>[2x]MTHSQQSMVDTFRASLFDNQDITVADQQIQALPYSTMYLRLNEGQRIFVVLGYIEQEQSKWLSQDNAM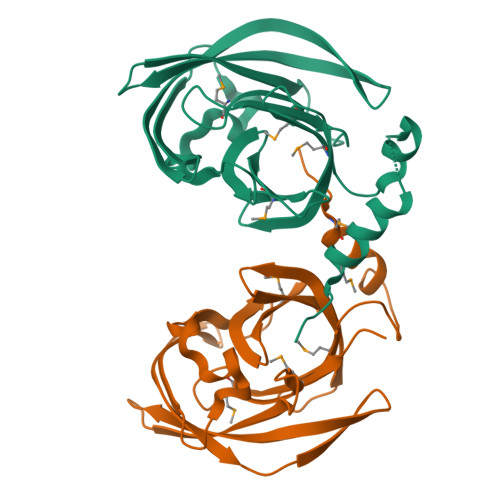LVTHNGRLLKTVKLNNNLLEVTNSGQDPLRNALAIKDGSRWTRDILWSEDNHFRSATLSSTFSFAGLETLNIAGRNVLCNVWQEEVTSTRPEKQWQNTFWVDSATGQVRQSRQMLGAGVIPVEMTFLKPAPLEHHHHHH> VVRILGGKARGVALKVPASARPSPVRLRKALFDYLRLRYPRRGRFLDPFAGSGAVGLEAASEGWEAVLVEKDPEAVRLLKENV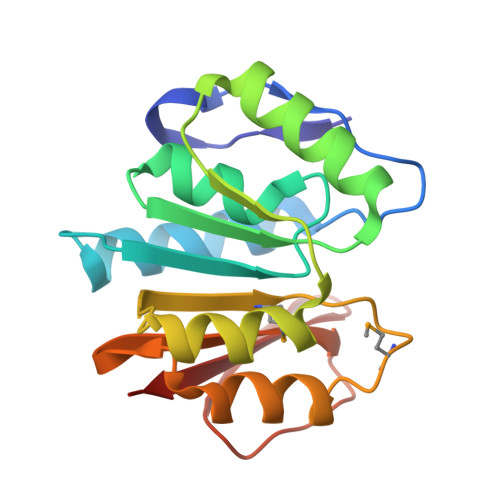RRTGLGARVVALPVEVFLPEAKAQGERFTVAFMAPPYAMDLAALFGELLASGLVEAGGLYVLQHPKDLYLPLGERRVYGENALTLVEV>MHHHHHHGARIIYDRAFLMACRGGGGENLYFQGKHPLQNRWALWFFKNDKSKTWQANLRLISKFDTVEDFWALYNHIQLSSNLMPGCDYSLFKDGIEPMWEDEKNKRGGRWLITLNKQQRRSDLNRFWLETLLCLIGESFDDYSDDVCGAVVNVRAKGDKIAIWTTECENREAVTHIGRVYKERLGLPPKIVIGYQSHADTATKSGSTTKNRFVV[2x]

Eukaryotic initiation factor 4E (eIF4E) serves as a regulatory hub for oncogene-driven protein synthesis and is considered a promising anticancer target. The eIF4F complex includes a core of eIF4E, eIF4G and eIF4A5,6. eIF4E recognises and binds the mRNA 5’cap, and recruits eIF4G to provide a scaffold function for the eIF4F complex, while eIF4A is an RNA helicase that is stimulated by binding to eIF4E and eIF4G8. Here we screen a fragment library against eIF4E and identify a ligand-binding site with previously unknown function.

The biaryl compound 1 binds site 2 in an enclosed hydrophobic cavity bounded by residues from the α1 and α2 helices and the β1, 2 and 3 sheets, plus a loop region linking the C-terminus of the α1 helix with the N-terminus of the β3 sheet. The binding of compound 1 appears to be driven primarily by hydrophobic van der Waals contacts and does not make any direct polar interactions with the protein. Isothermal titration calorimetry (ITC) indicated that the binding affinity (Kd) of 1 for eIF4E was 400 µM with reasonable ligand efficiency (LE 0.36). Initial optimisation of compound 1 focused on more efficiently filling the hydrophobic cavity and growing from the 4-position of the biphenyl to understand the structural requirements for inducing the loop movement.> EAEAGNDLLSCLTFNGVRNHTVFSADSDSDFNRFLHLSIQNPLFQNSLISKPSAIILPGSKEELSNTIRCIRKGSWTIRLRSGGHSYEGLSYTSDTPFILIDLMNLNRVSIDLESETAWVESGSTLGELYYAITESSSKLGFTAGWCPTVGTGGAISGGGFGMMSRKYGLAADNVVDAILIDANGAILDRQAMGEDVFWAIRGGGGGVWGAIYAWKIKLLPVPEKVTVFRVTKNVAIDEATSLLHKWQFVAEELEEDFTLSVLGGADEKQVWLTMLGFHFGLKTVAKSTFDLLFPELGLVEEDYLEMSWGESFAYLAGLETVSQLNNRFLKFDERAFKTKVDLTKEPLPSKAFYGLLERLSKEPNGF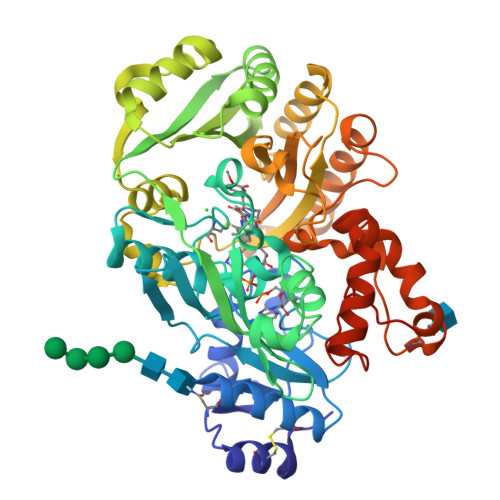IALNGFGGQMSKISSDFTPFPHRSGTRLMVEYIVAWNQSEQKKKTEFLDWLEKVYEFMKPFVSKNPRLGYVNHIDLDLGGIDWGNKTVVNNAIEISRSWGESYFLSNYERLIRAKTLIDPNNVFNHPQSIPPMANFDYLEKTLGSDGGEVVI>MVKVHF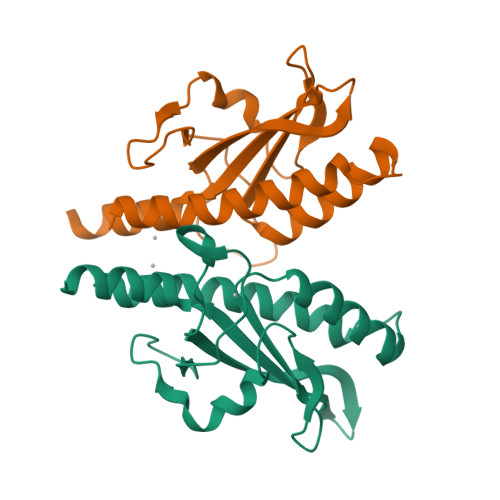AEQDINDLKEISATLERVLNHPDETQARRLMTLEDIVSGYSNVLISLADSQGKTVYHSPGAPDIREFTRDAIPDKDAQGGEVYLLSGPTMMMPGHGHGHMEHSNWRMINLPVGPLVDGKPIYTLYIALSIDFHLHYINDLMNKL[4x]> GLPVLNTPGSNQYLTADNYQSPCAIPEFDVTPPIDIPGEVRNMMELAEIDTMIPLNLTNQRKNTMDMYRVELNDAAHSDTPILCLSLSPASDPRLAHTMLGEILNYYTHWAGSLKFTFLFCGSMMATGKLLVSYAPPGAEAPKSRKEAMLGTHVIWDIGLQSSCTMVVPWISNTTYRQTINDSFTEGGYISMFYQTRVVVPLSTPRKMDILGFVSACNDFSVRLLRDTTHI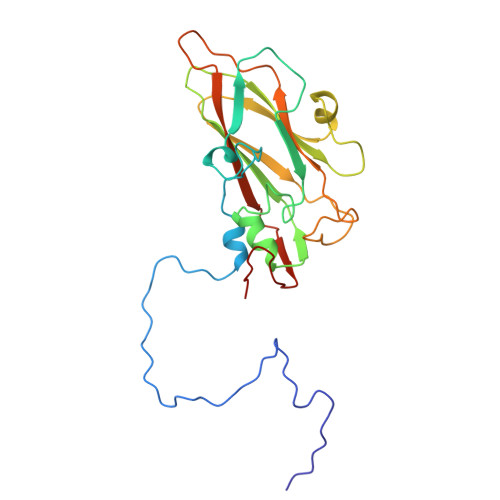SQEAMPQ>[2x]GAMNAQAEEFKKYLETNGIKPKQFHKKELIFNQWDPQEYCIFLYDGITKLTSISENGTIMNLQYYKGAFVIMSGFIDTETSVGYYNL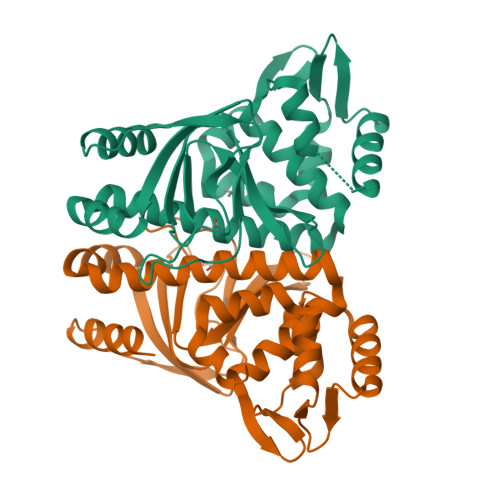EVISEQATAYVIKINELKELLSKNLTHFFYVFQTLQKQVSYSLAKFNDFSINGKHGSICGQLLILTYVYGKETPDGIKITLDNLTMQELGYSSGIAHSSAVSRIISKLKQEKVIVYKNSCFYVQNLDYLKRYAPKLDEWFYLACPATWGKLN> MDIEFTTSAASQASLPRGRRTARPSGDDRELAILATAENLLEDRPLADISVDDLAKGAGISRPTFYFYFPSKEAVLLTLLDRVVNQADMALQTLAENP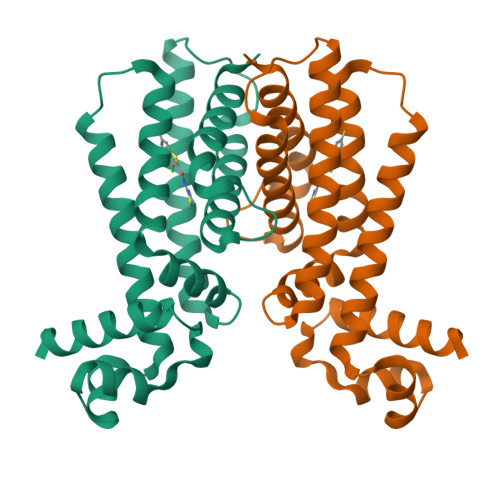ADTDRENMWRTGINVFFETFGSHKAVTRAGQAARATSVEVAELWSTFMQKWIAYTAAVIDAERDRGAAPRTLPAHELATALNLMNERTLFASFAGEQPSVPEARVLDTLVHIWVTSIYGENRGSHHHHHH> MGPYLQILEQPKQRGFRFRYVCEGPSHGGLPGASSEKNKKSYPQVKICNYVGPAKVIVQLVTNGKNIHLHAHSLVGKHCEDGVCTVTAGPKDMVVGFANLGILHVTKKKVFETLEARMTEACIRGYNPGLLVHSDLAYLQAEGGGDRQLTDREKEIIRQAAVQQTKEMDLSVVRLMFTAFLPDSTGSFTRRLEPVVSDAIYDSKAPNASNLKIVRMDRTAGCVTGGEEIYLLCDKVQKDDIQIRFYEEEENGGVWEGFGDFSPTDV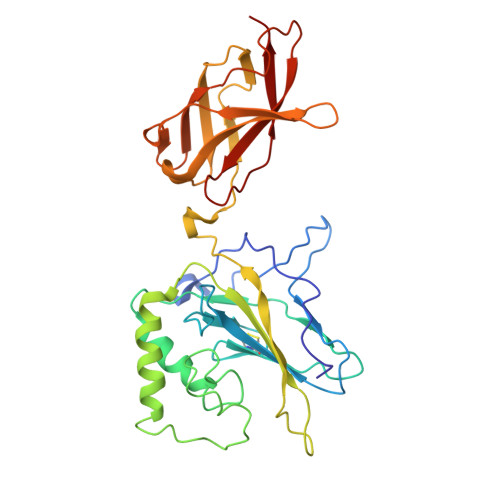HRQFAIVFKTPKYKDVNITKPASVFVQLRRKSDLETSEPKPFLYYPE>[5x]AQDMVSPPPPIADEPLTVNTGIYLIECYSLDDKAETFKVNAFLSLSWKDRRLAFDPVRSGVRVKTYEPEAIWIPEIRFVNVENARDADVVDISVSPDGTVQ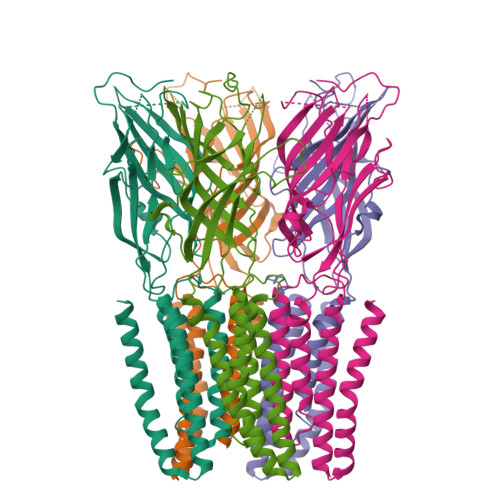YLERFSARVLSPLDFRRYPFDSQTLHIYLIVRSVDTRNIVLAVDLEKVGKNDDVFLTGWDIESFTAVVKPANFALEDRLESKLDYQLRISRQYFSYIPNIILPMLFILFISWTAFWSTSYEANVTLVVSTLIAHIAFNILVETNLPKTPYMTYTGAIIFMIYLFYFVAVIEVTVQHYLKVESQPARAASITRASRIAFPVVFLLANIILAFLFFGF5-phenylthiophene-2-carboxylic acid | C11 H8 O2 S | 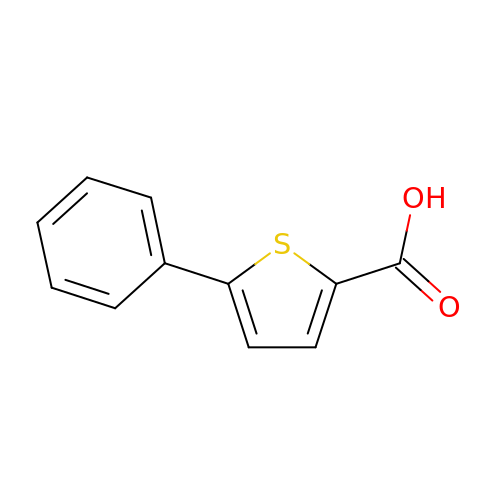QGMFBCDNJUZQBZ-UHFFFAOYSA-N>[2x]AMNYFVGNSLGVNLTGIEKAIINRLNLFKEMGRPAQCVFLSWNRYLYRNAQNYITSSDYINMYDFFQEATYLERNEPFDWLSYWTDECHYTLKHVENSHDFRIYDQERFLMYAHFQDPKYRILDYVNHFDSQRRKVKRDFYDVRGFLSCSRILVDKQQTLCEFFYNPEGDTKLEKYFSYKDGKPEVQKIIVYYANKQYFFNNETELGAFFIKQLYQHGDLFFSDRNVYTAPIFNLTPESIPVVAVLHSTHIKNIDALDSSPFKNVYKAMFENLSRYRAIIVSTEQQKLDVEKRINHTIPVVNIPVGYSETIDTPVQTLDQRSVKLISVARYSPEKQLHQQIELIKRLVSYVPKIELHMYGFGSESKKLNELIQKYGLENHVYLRGFLSNLDQEYSDAYLSLITSNMEGFSLALLESLAHGVPVISYDIKYGPNELITSDFNGYLITKNDEDALFDKVKYVIDHPEVQQRLSKGSLAKAQQYSKASLIKQWDQFVRLILEHHHHHH;>SDSDSDSD[2x]

Two glycosyltransferases (GTases), SdgB and SdgA, are responsible for the glycosylation of S. aureus SDR proteins such as ClfA and ClfB. SdgB first appends N-acetyl­glucosamine (GlcNAc) moieties onto serine residues (O-glycosylation) within the SDR domain using uridine diphos­phate N-acetylglucosamine (UDP-GlcNAc) as a donor substrate. The subsequent addition of GlcNAc to the glycoproteins is catalyzed by the second enzyme, SdgA, yielding glycosylated SDR proteins in which each SD repeat is decorated with GlcNAc disaccharide moieties. The glycosylation of SDR proteins mediated by SdgA and SdgB protects SDR proteins from degradation by host proteases, thereby circumventing innate immune attack.

Despite the biological significance of these two glycosyltransferases involved in pathogenicity and avoidance of the host innate immune response, their structures and the molecular basis of their activity have not been investigated. This study reports the crystal structures of SdgB and SdgA from S. aureus as well as multiple structures of SdgB in complex with its substrates (for example UDP, N-acetylglucosamine or SDR peptides), products (glycosylated SDR peptides) or phosphate ions. Interestingly, SdgB undergoes a conformational change from an open to closed complex upon substrate binding. In addition to the dimerization role, the inserted domain was found to serve as a binding platform for the SD repeats before and after glycosylation. A long positive tract along the inserted domain stabilizes the binding of the glycosylated SD repeats to SdgB by offsetting the negative charge clustered in the tandem SD repeats. SdgB and SdgA share the way that they recognize monoglycosylated SD repeats as a product and a substrate, respectively, but SdgA is likely to preferentially bind a longer SDR substrate than a shorter one.> MTATVLLEVPFSARGDRIPDAVAELRTREPIRKVRTITGAEAWLVSSYALCTQVLEDRRFSMKETAAAGAPRLNALTVPPEVVNNMGNIADAGLRKAVMKAITPKAPGLEQFLRDTANSLLDNLITEGAPADLRNDFADPLATALHCKVLGIPQEDGPKLFRSLSIAFMSSADPIPAAKINWDRDIEYMAGILENPNITTGLMGELSRLRKDPAYSHVSDELFATIGVTFFGAGVI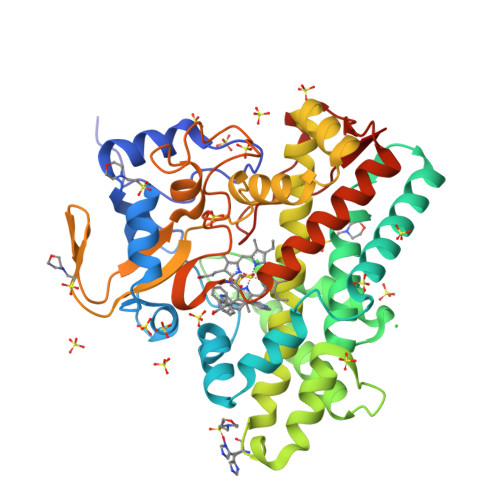STGSFLTTALISLIQRPQLRNLLHEKPELIPAGVEELLRINLSFADGLPRLATADIQVGDVLVRKGELVLVLLEGANFDPEHFPNPGSIELDRPNPTSHLAFGRGQHFCPGSALGRRHAQIGIEALLKKMPGVDLAVPIDQLVWRTRFQRRIPERLPVLW>[2x]AERENLKNEATKVLEHVCEDINKESYGFVKISKMKENEKEIRLFNLEEIYHSLMKVGGSGATDGGKREDDAASHSVVAESNGAHLLQSDIWVRGRIHDIRSKGSLAFIILRHKLYSMQCILDIKHNDNDKNMMKWVSNLPLESIVDIKGKLSKPEVPID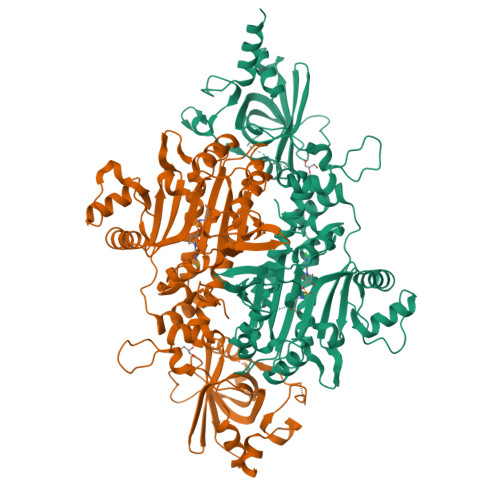STNIKYEAHIRKIFCISKTAKELPFLLKDANMKETNEEGSIKVNQDNRLNNRCVDLRTYANYSIFCLQSQICTIFKNFLLENNFIEIHTPKLLGESSEGGANAFQINYFNQKGFLAQSPQLYKQMCINSGFDRVFEVAPVFRAENSNTYRHLCEYVSLDVEMTYKYDYLENVHFYDSMFKHIFTELSKGGKNEMLIKTVKGQYPCEDFQWLEETPIFTYEEAIKMLIQHGKLHLKEEEILAYDMSTDMEKELGKIVKASHHTDYYIIINFPSALRPFYTMYKEDEPAISNSYDFFMRGEEILSGSQRISDVNLLLENIKRFNLDANKLNFYIDSFAYSSYPHSGCGIGLERVLMLFLGLNNIRKTSLFPRDPKRLIP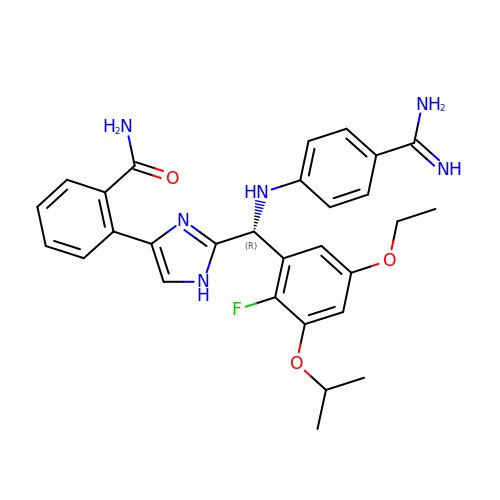2-[2-[(R)-[(4-carbamimidoylphenyl)amino]-(5-ethoxy-2-fluoranyl-3-propan-2-yloxy-phenyl)methyl]-1H-imidazol-4-yl]benzamide | C29 H31 F N6 O3 | KAQSSNYVMPKBOO-AREMUKBSSA-N>MGHHHHHHENLYFQGVQKIGILGAMREEITPILELFGVDFEEIPLGGNVFHKGVYHNKEIIVAYSKIGKVHSTLTTTSMILAFGVQKVLFSGVAGSLVKDLKINDLLVATQLVQHDVDLSAFDHPLGFIPESAIFIETSGS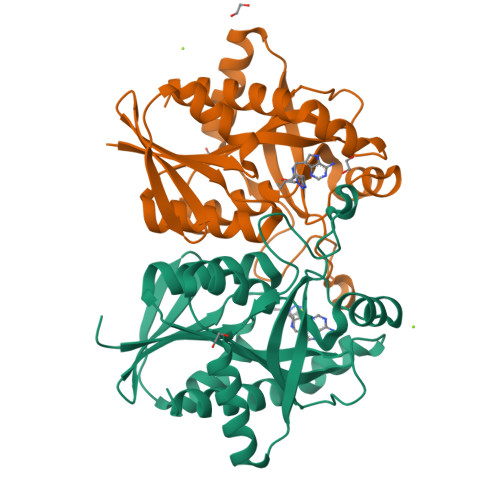LNALAKKIANEQHIALKEGVIASGDQFVHSKERKEFLVSEFKASAVEMEGASVAFVCQKFGVPCCVLRSISDNADEKAGMSFDEFLEKSAHTSAKFLKSMVDEL[4x]> EDKYTDKYDNINLDEILANKRLLVAYVNCVMERGKCSPEGKELKEHLQDAIENGCKKCTENQEKGAYRVIEHLIKNEIEIWRELTAKYDP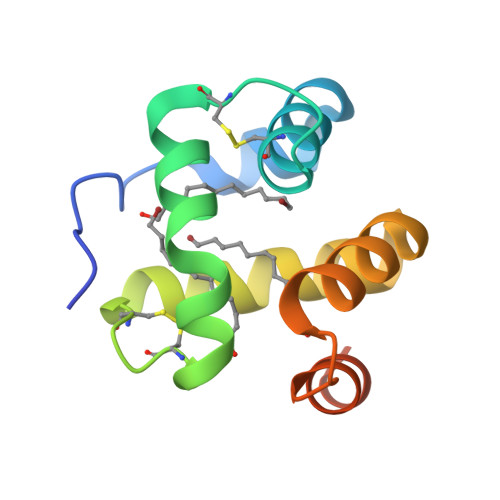TGNWRKKYEDRAKAAGIVIPEE>MENLIGYVAAFLTTVSFLPAVLRVVMTKQTRDISRNMYIMFFLGVVLWFVYGILRSDLPIILANV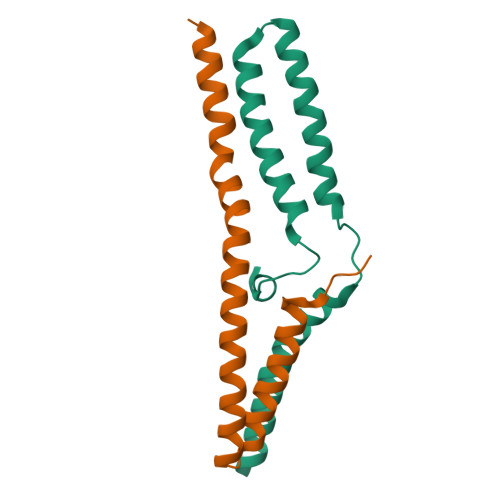VTLFFVTIILYYKLTEGNQTGSLEVLFQ[4x]>[2x]GHMDMQHRIRQLFQASIETKQQALEVLPPYIEQASLVMVNALLNEGKILSC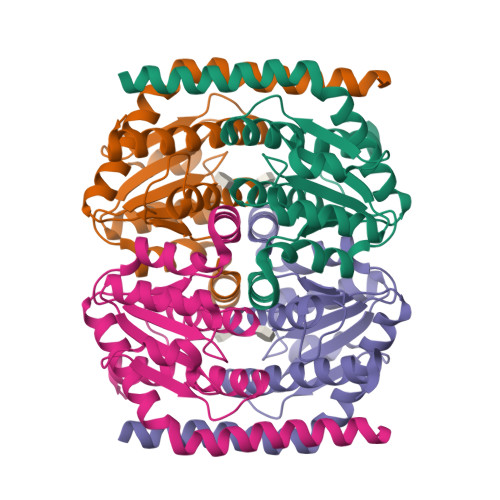GNGGSAGDAQHFSSELLNRFERERPSLPAVALTTDSSTITSIANDYSYNEVFSKQIRALGQPGDVLLAISTSGNSANVIQAIQAAHDREMLVVALTGRDGGGMASLLLPEDVEIRVPSKITARIQEVHLLAIHCLCDLIDRQLFGSEE> AVSFIGSTENDVGPSLGSYSRTHAMDNLPFVYDTRNKIGYQNANVWHISKGFCVGLDGKVDLPVVGSLDGQSIYGLTEEVGLLIWMGDTKYSRGTAMSGNSWENVFSGWCVGANTASTQGLSVRVTPVILKRNSSSRYSVQKTSIGSIRMRPYN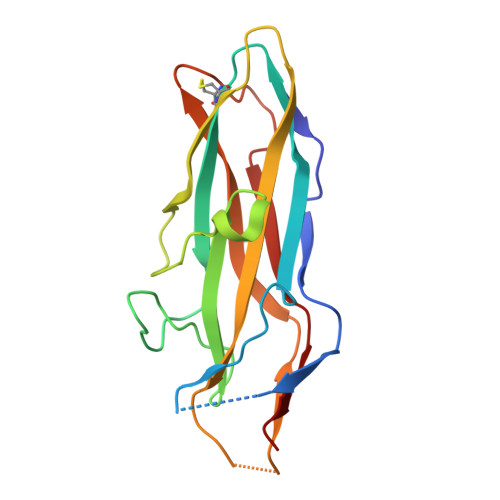GSSAGSVQTTVNFSLNPFTLNDT>[4x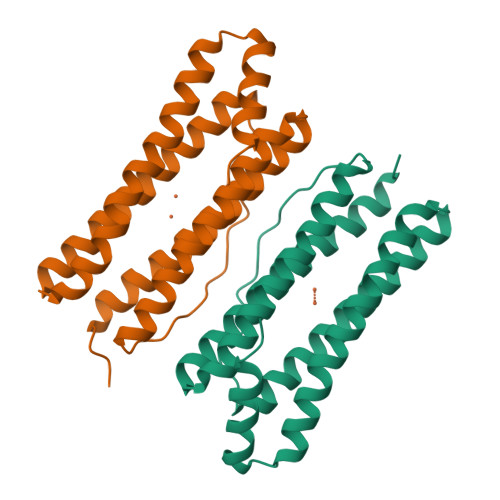]MMVISEKVRKALNDQLNREIYSSYLYLSMATYFDAEGFKGFAHWMKKQAQEELTHAMKFYEYIYERGGRVELEAIEKPPSNWNGIKDAFEAALKHEEFVTQSIYNILELASEEKDHATVSFLKWFVDEQVEEEDQVREILDLLEKANGQMSVIFQLDRYLGQRE> RHRK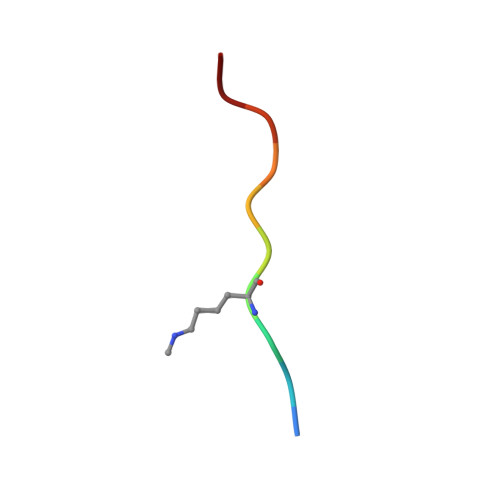VLRDNY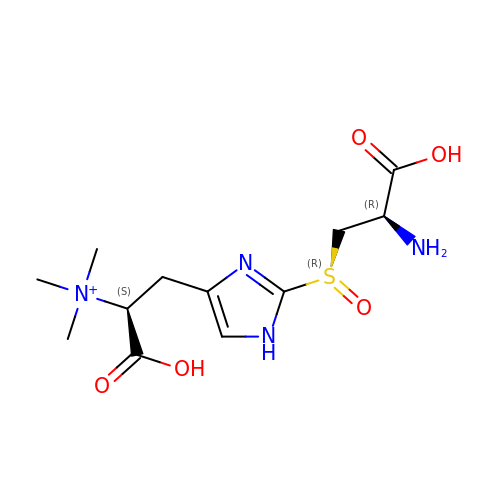(1S)-2-{2-[(R)-(2R)-2-amino-2-carboxyethanesulfinyl]-1H-imidazol-4-yl}-1-carboxy-N,N,N-trimethylethan-1-aminium | C12 H21 N4 O5 S | CSTNDZVKJNPMIG-YWHIBEFZSA-O> DNNVLLTGDVIHTDNQLSYESAAFVMQGDCN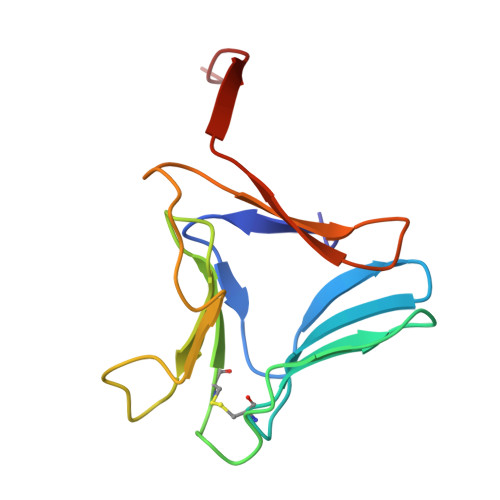LVLYNEAGGFQSNTHGRGVDCTLRLNNRGQLEIHSANSNTPVWVYPRSVNTVRGNYAATLGPDQHVTIYGPAIWSTPAAA>[2x]MTIPTLYMNDGMNAQSSQALHIQTYCNSVRQQIPVDFGRFPNLRESERQINTGLGAARQHAEHYLKDIQPLIIRNVTNIQDYFETQNLISTVMPSGATKEQWLSALGMVSDKAKEYQEVSANTRRTIGSLNDKLIIDSNNYQLIVVNLNNVVNGNNGVLEQLNRD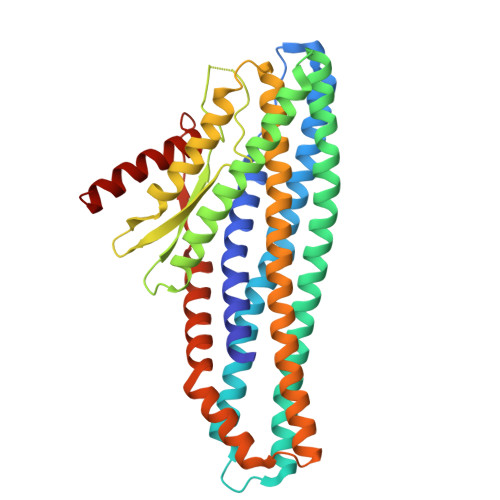IDGINAAIDGAIAGIVVGGLLVIGGAIVTAIGAVAGLVTAGTSTPVVMGGIAMMTAGAGGVIGGAIVLDKSLSAREKLYRDRSQLNSEVLVASQIGSGYRGLQTQAQSAVTAATQMNNAWDSLTSELETLNANLRKGIIDDSFLRQLFLTASQTSVTKVLDGTKIIKQQMAGVVVREVPANQSIADFVKRLAALEHHHHHH>[2x]AAPTAIEHMEPPFWWAGMQHKGLQLMVHGRDIGRMEAALDYPGVRLVSPTRVPNANYLFVDLEIGPEAQPGSFDIVFKGDGRSERYRYRLLAREQGSAQRQGFGPGDAIYQIMPDRFANGDPSNDNVAGMREQADRRHGGGRHGGDIRGTIDHLDYIAGLGFTQLWPTPL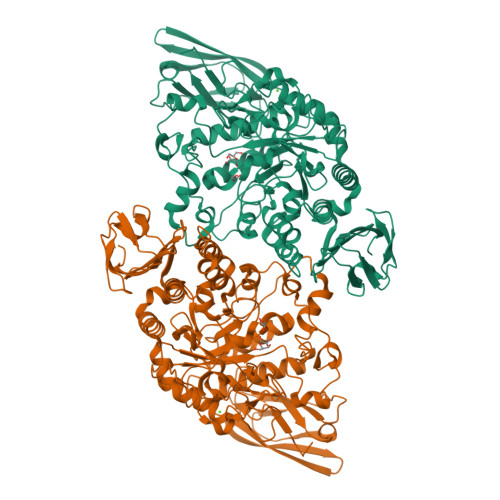VENDAAAYSYHGYAATDHYRIDPRYGSNEDFVRLSTEARKRGMGLIQDVVLSHIGKHHWWMKDLPTPDWINYGGKFVPTQHHRVAVQDPYAAQADSENFTKGWFVEGMPDLNQTNPLVANYLIQNNIWWIEYAGLSGLRIDTYGYSDGAFLTEYTRRLMAEYPRLNMVGEEWSTRVPVVARWQRGKANFDGYTSHLPSLMDFPLVDAMRNALSKTGEENGLNEVYETLSLDYLYPEPQNLVLFGGNHDMARMFSAAGEDFDRWRMNLVFLMTMPRIPQFYSGDEILMTSTVKGRDDASYRRDFPGGWAGDKANAFSGAGLTSQQRAAQDLVRKLANWRKNQPVIHNGRLMHFGPEENTWVYFRYNKDKRIMVAMNNNDKPMTLPTARFQEMLKGAPSGVDFLSGKTVGLGRELRLAPKSVVVIELPGLPEA>MEHSEMKMSDMHSSASSQEYMAGMKNMHEKMMAAVNESNPDKAFAKGMIAHHEGAIAMAETELKYGKDPEMRKLAQDIIKAQKGEIEQMNKWLDSHKLEHHH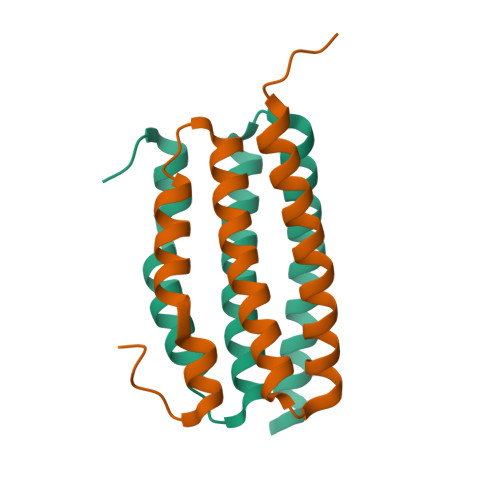HHH[2x]> QGFSLAQYLQEQKTIVETALDQSLVITEPVTIYEAMRYSLLAGGKRLRPILCLAACEMLGGTAAMAMNTACALEMIHTMSLIHDDLPAMDNDDLRRGKPTN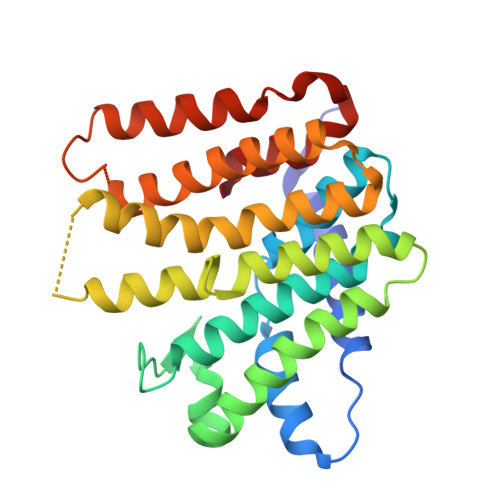HKVYGEDIAILAGDALLSYAFEYVARTPDVPAERLLQVIVRLGQAVGAEGLVGGQVVDLESEGVETLNFIHTHKTGALLEVCVTAGAILAGAKPEEVQLLSRYAQNIGLAFQIVDDILLWGIEKSQAEAQKLVAEAIASLEPYGEKANPLKALAEYI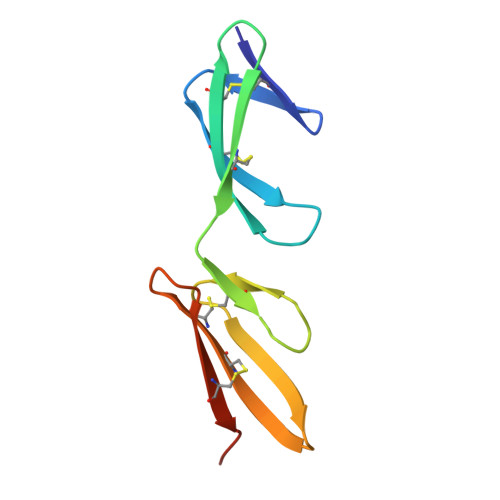> DQCIVDDITYNVQDTFHKKHEEGHMLNCTCFGQGRGRWKCDPVDQCQDSETGTFYQIGDSWEKYVHGVRYQCYCYGRGIGEWHCQPLQTYPSS Phosphite dehydrogenase (PTDH), first discovered in Pseudomonas stutzeri WM88, catalyzes the oxidation of phosphite to phosphate, which is coupled to the reduction of NAD+ to NADH. The enzyme follows an ordered kinetic mechanism with NAD+ binding before phosphite. The crystal structure of 17X-PTDH indicates that Arg301 is situated at the dimer interface, but its side chain orients inwards towards the enzyme active site. As such, Arg301 is in position to directly affect catalysis, through either electrostatic interactions if it is in the guanidinium form, or by acting as a catalytic base to deprotonate a water molecule if the guanidine is deprotonated.

The 2.35 Å resolution crystal structure of the R301A mutant with NAD+ bound shows that removal of the guanidine group renders the active site solvent exposed, suggesting the possibility of chemical rescue of activity. Crystals were obtained that contained NAD+ and that diffracted to 2.35 Å and 2.65 Å for the R301A and R301K mutants, respectively. Comparison of the 17X-PTDH and R301A X-ray structures, both with NAD+ bound, shows that the mutant has a solvent exposed phosphite binding site that is covered by the side chain of Arg301 in the wild type structure. The multifaceted but incompletely understood role of Arg301 combined with the solvent-exposed active site in the R301A mutant prompted attempts of chemical rescue experiments to better define the function or Arg301. The poor activity of the R301A mutant could indeed be markedly improved by addition of exogenous guanidine, methylguanidine, acetamidine, aminoguanidine, ethylguanidine, or N-guanylurea. We show that the catalytic activity of this mutant is restored to near wild-type levels by the addition of exogenous guanidinium analogues; Brønsted analysis of the rates of chemical rescue suggests that protonation of the rescue reagent is complete in the transition state of the rate-limiting step. In addition, sulfite inhibition studies showed a large increase in the dissociation constant for binding with the R301A mutant, and sulfite binding could not be substantially improved by addition of rescue agent. Collectively, these findings along with the X-ray structures illustrate that proper positioning of the side chain of Arg301 is very important for efficient capturing of phosphite, which cannot be recapitulated by the rescue agents for the R301A variant.

>[2x]MLPKLVITHRVHEEILQLLAPHCELITNQTDSTLTREEILRRCRDAQAMMAFMPDRVDADFLQACPELRVIGCALKGFDNFDVDACTARGVWLTFVPDLLTVPTAELAIGLAVGLGRHLRAADAFVRSGKFRGWQPRFYGTGLDNATVGFLGMGAIGLAMADRLQGWGATLQYHAAKALDTQTEQRLGLRQVACSELFASSDFILLALPLNADTLHLVNAELLALVRPGALLVNPCRGSVVDEAAVLAALERGQLGGYAADVFEMEDWARADRPQQIDPALLAHPNTLFTPHIGSAVRAVALEIERCAAQNILQALAGERPINAVNRLP> GSGVPINVKCRGSRDCLDP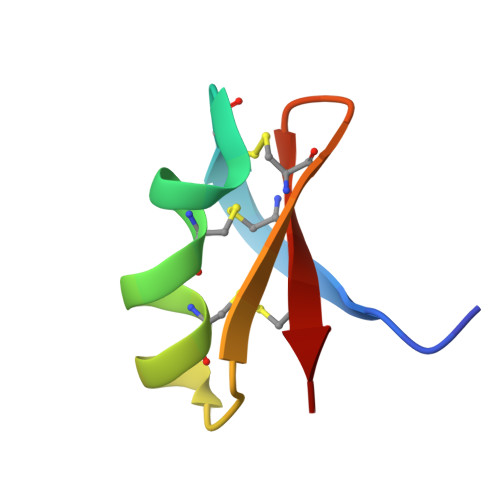CKKAGMRFGKCINSKCHCTP>[2x]VLAQNKADVISKCLDDAGIRNVIDTDSSWAQETVMFQKRLKPDPEAIAFPENSDEVASALKCARESKVK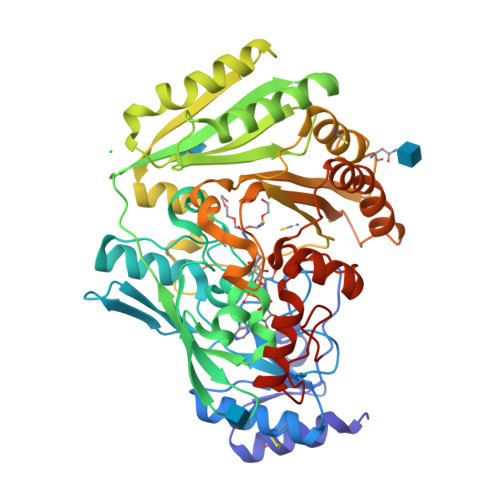ANALGPAHSFQGNGFGIPGNLVINMAAFDEVSYDKKSTLLTFGGGTHVGPVQKYLWDTAGRHVPHVRGAHVGVTGSSIGGGFGTTSRYLGTPMDNLVEIQYMLYNGTIVNAKKGSDLFWAAQGAGASFGIILSTKTKTFKPQFDKAINFTLSMGDLTPEAGAKALVAIQDYSLSKDCPDTWAFRWNIMAPPYDGTGYFYGNPSSFDSVMAPLVKKLKTISSNTAVKSTVLPWWDLEVAVAGPGMNQPNGGALGGRSFYTQSLTTTTDHPLTVKQAQILFEGTTLAFNRTDMTKFGYMDLWGGVSRSIKDSDTAYAHGKNLWLIRWDANAIGAYPSDGISYMRASIKPFEDSLVKGGAKLRGFVNYADTELTEKEWSSRLYDGNFERLKQIKARYDPEGLFINHRQSIPLPAAAHHHHHH> GIDPFTGLSSDKIDEMYDIFGDGHDYDWALEIENEELENGNDNNEAEEEEIDEETGAIKSTKKKISLQDIYDLEDLKKNLMTEGDMKIRKTDIPERYQELRAGITDYGNMSSEDQELERNWIAEKISVDKNFDANYDLTEFKEAIGNAIKFITKENLEVPFIYAYRRNYISSREKDGFLLTEDDLWDIVSLDIEFHSLVNKKDYVQRFYAELHIDDPIVTEYFKNQNTA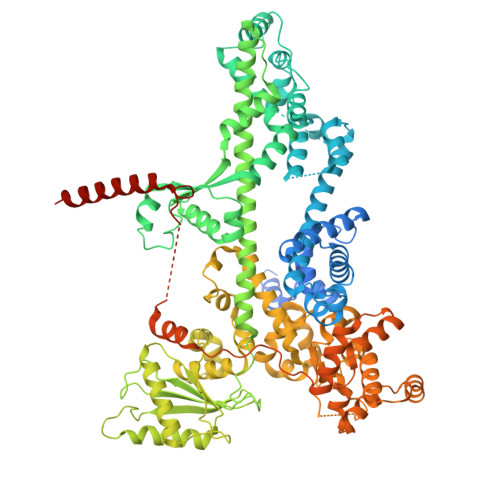SIAELNSLQDIYDYLEFKYANEINEMFINHTGKTGKKHLKNSSYEKFKASPLYQAVSDIGISAEDVGENISSQHQIHPPVDHPSSKPVEVIESILNANSGDLQVFTSNTKLAIDTVQKYYSLELSKNTKIREKVRSDFSKYYLADVVLTAKGKKEIQKGSLYEDIKYAINRTPMHFRRDPDVFLKMVEAESLNLLSVKLHMSSQAQYIEHLFQIALETTNTSDIAIEWNNFRKLAFNQAMDKIFQDISQEVKDNLTKNCQKLVAKTVRHKFMTKLDQAPFIPNVRDPKIPKILSLTCGQGRFGADAIIAVYVNRKGDFIRDYKIVDNPFDKTNPEKFEDTLDNIIQSCQPNAIGINGPNPKTQKFYKRLQEVLHKKQIVDSRGHTIPIIYVEDEVAIRYQNSERAAQEFPNKPPLVKYCIALARYMHSPLLEYANLTSEEVRSLSIHPHQNLLSSEQLSWALETAFVDIVNLVSVEVNKATDNNYYASALKYISGFGKRKAIDFLQSLQRLNEPLLARQQLITHNILHKTIFMNSAGFLYISWNEKRQKYEDLEHDQLDSTRIHPEDYHLATKVAADALEYDPDTIAEKEEQGTMSEFIELLREDPDRRAKLESLNLESYAEELEKNTGLRKLNNLNTIVLELLDGFEELRNDFHPLQGDEIFQSLTGESEKTFFKGSIIPVRVERFWHNDIICTTNSEVECVVNAQRHAGAQLRRPANEIYEIGKTYPAKVIYIDYANITAEVSLLDHDVKQQYVPISYSKDPSIWDLKQELEDAEEERKLMMAEARAKRTHRVINHPYY>MTSAEMTSPNNNSEHQAIAKMRTMIEGFDDISHGGLPIGRSTLVSGTSGTGKTLFS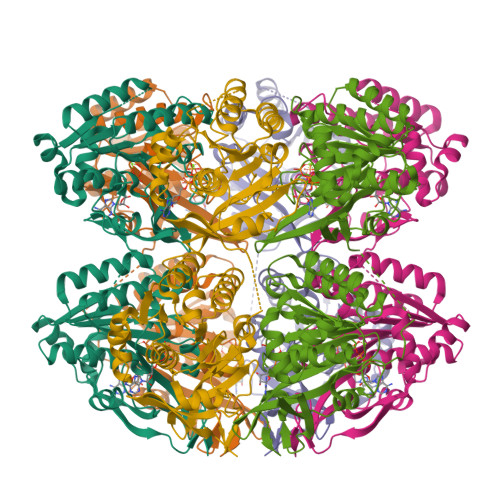IQFLYNGIIEFDEPGVFVTFEETPQDIIKNARSFGWDLAKLVDEGKLFILDASPDPEGQEVVGGFDLSALIERINYAIQKYRARRVSIDSVTSVFQQYDASSVVRRELFRLVARLKQIGATTVMTTERIEEYGPIARYGVEEFVSDNVVILRNVLEGERRRRTLEILKLRGTSHMKGEYPFTITDHGINIFPLGAMRLTQRSSNVRVSSGVVRLDEMCGGGFFKDSIILATGATGTGKTLLVSRFVENACANKERAILFAYEESRAQLLRNAYSWGMDFEEMERQNLLKIVCAYPESAGLEDHLQIIKSEINDFKPARIAIDSLSALARGVSNNAFRQFVIGVTGYAKQEEITGLFTNTSDQFMGAHSITDSHISTITDTIILLQYVEIRGEMSRAINVFKMRGSWHDKAIREFMISDKGPDIKDSFRNFERIISGSPTRITVDEKSELSRIVRGVQEKGPES[2x]> SATRANKDIFTLFDKKGQGAIAKDSLGDYLRAIGYNPTNQLVQDIINADSSLRDASSLTLDQITG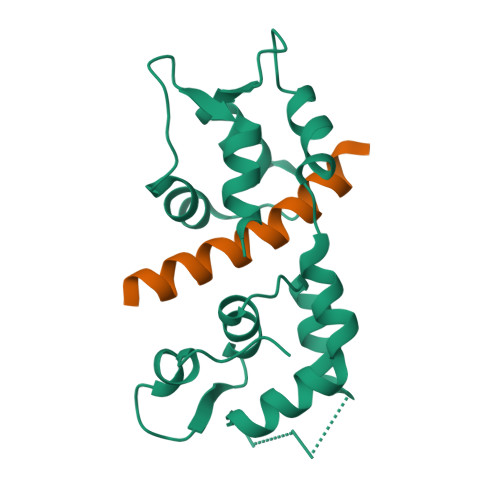LIEVNEKELDATTKAKTEDFVKAFQVFDKESTGKVSVGDLRYMLTGLGEKLTDAEVDELLKGVEVDSNGEIDYKKFIEDVLRQ;> QISQAIKYLQNNIKGFIIRQRVNDE>LQGRIAASADAQLELIGPRAAAAASLESAVLHVSLTARAYALTPEPARMDALQAALRRLEGAAARFAALPKSPEGAALSGRILAAVPPFEKAAVALGTAVATGGDDSAIRAREATLPPMREELLSLLRTFGALQQAHDAGASHTILAYQRDT[2x]

Many of the HK and MCP signal transduction proteins span the cytoplasmic membrane and detect extracytoplasmic signals/stimuli via “sensor” domains that face the periplasm. Binding of a small molecule or other stimulus to these domains initiates a response in the cytoplasmic domains, which in turn triggers the downstream regulatory processes. We have undertaken a study of the periplasmic sensor domains from A. dehalogenans 2CP-C with an eventual goal of delineating the functions of some of the signal transduction proteins (The term “signal transduction proteins” hereafter is used to refer to transmembrane sensor histidine kinases [HK] and methyl-accepting chemotaxis [MCP] proteins only) from this organism. Although sensor domains have been studied for many years, there are still many unknowns about the actual ligands that stimulate a given response and the mechanism of signal transduction. It is now apparent that both HK and MCP proteins interchangeably use the PAS-like (including tandem PAS-like) and helical bundle sensor domain tertiary folds.

Periplasmic sensor domain (residues 33–184) of chemotaxis protein Adeh_2942 was isolated, purified, and crystallized as described in the methods section. Adeh_2942 crystallized in space group C2 and diffracted X-rays to 2 Å resolution. Structure was determined by SAD method utilizing the selenomethionine residues and refined to an R-factor of 0.198 and R-free of 0.251. The sensor domain of Adeh_2942 crystallized as a head-to-tail dimer comprised of monomers that form up-down four-helix bundles. The four helices are formed by residues 38–75 (α1), 77–101 (α2), 104–134 (α3), and 137–179 (α4). The helices α1 and α4 have a kink at residues Glu46 and Ala146, respectively. The N- and C-termini of the sensor domain are juxtaposed so they can attach to the TM helices as expected in the full-length protein. In case of Adeh_2942 sensor, the crystallization process selected a head-to-tail dimer; in contrast the well-studied sensor domains of chemotaxis proteins, aspartate receptor, Tar, serine receptor, Tsr, and the nitrate sensing histidine kinase, NarX form head-to-head dimers that are considered physiologically relevant, and the ligand in each case is bound between the two monomers. The four-helix bundle structure of the monomer observed in Adeh_2942 is similar to that of Tar and Tsr sensor domains. Comparison of the monomer structure of Adeh_2942 sensor domain with that of Tar and Tsr has revealed a minor deviation from helical secondary structure in helix-4 (residues Ala146 and Thr147) in approximately similar location, however, the two prolines present in Adeh_2942 (residues 149 and 150) are within the helical secondary structure.4-(pyridin-3-yl)benzoic acid | C12 H9 N O2 | 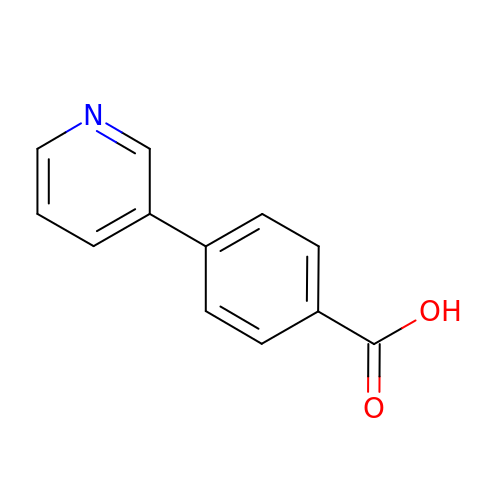GYUKEVKPDRXPAB-UHFFFAOYSA-N> SDVAF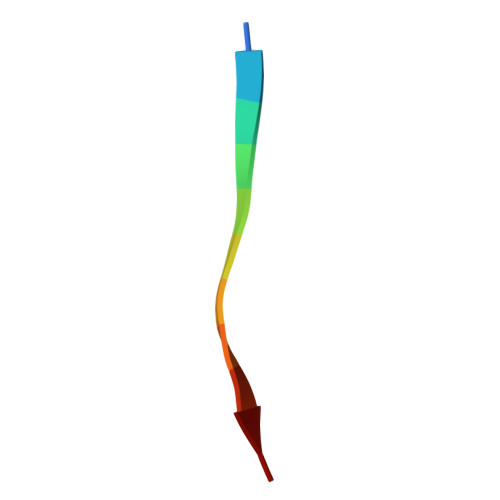RGNLLD> MKKGHHHHHHGSERTGTQPLGVQGLTEEQRMMIRELMDAQMKTFDTTFSHFKNFRLPGVLSSGCEL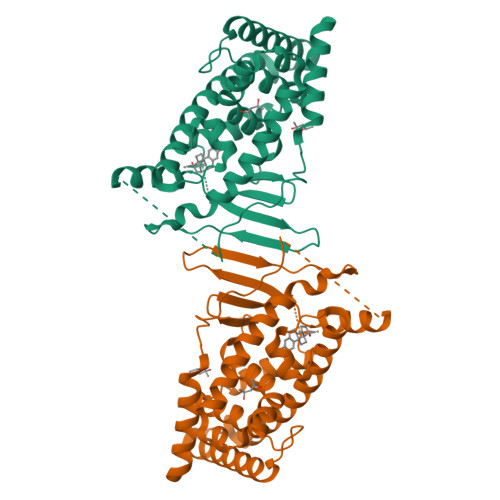PESLQAPSREEAAKWSQVRKDLCSLKVSLQLRGEDGSVWNYKPPADSGGKEIFSLLPHMADMSTYMFKGIISFAKVISYFRDLPIEDQISLLKGAAFELCQLRFNTVFNAETGTWECGRLSYCLEDTAGGFQQLLLEPMLKFHYMLKKLQLHEEEYVLMQAISLFSPDRPGVLQHRVVDQLQEQFAITLKSYIECNRPQPAHRFLFLKIMAMLTELRSINAQHTQRLLRIQDIHPFATPLMQELFGITGS> MKKIIYIAT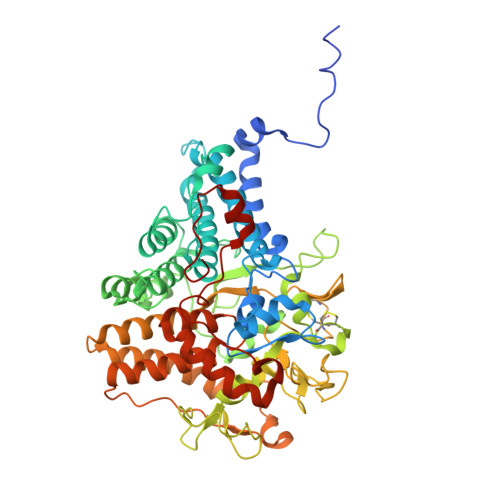IGITLLTTSCDDFLDRQVPQGIVTGDQIASPEYVDNLVISAYAIWATGDDINSSFSLWNYDVRSDDCYKGGSGTEDGGVFNALEISKGINTTDWNINDIWKRLYQCITRANTALQSLDQMDEKTYPLKNQRIAEMRFLRGHAHFMLKQLFKKIVIVNDENMEPDAYNELSNTTYTNDEQWQKIADDFQFAYDNLPEVQIEKGRPAQAAAAAYLAKTYLYKAYRQDGADNALTGINEEDLKQVVKYTDPLIMAKGGYGLETDYSMNFLPQYENGAESVWAIQYSINDGTYNGNLNWGMGLTTPQILGCCDFHKPSQNLVNAFKTDSQGKPLFSTYDNENYEVATDNVDPRLFHTVGMPGFPYKYNEGYIIQKNDDWSRSKGLYGYYVSLKENVDPDCDCLKKGSYWASSLNHIVIRYADVLLMRAEALIQLNDGRITDAISLINEVRSRAAGSTMLIFNYKEDYGVNFKVTPYDLKAYAQDEAMKMLKWERRVEFGMESSRFFDLVRWGEAKDVINAYYVTEASRCSIYKNAGFTENKNEYLPVPFEQISASNGNYTQNFGWHHHHHH>MKRKLFWICAVAMGMSAFPSFMTQATPATQPLINAEPAVAAQTEQNPQVGQVMPGVQGADAPVVAQNGPSRDVKLTFAQIAPPPGSMVLRGINPNGSIEFGMRSDEVVTKAMLNLEYTPSPSLLPVQSQLKVYLNDELMGVLPVTKEQLGKKTLAQMPINPLFITDFNRVRLEFVGHYQDVCENPASTTLWLDVGRSSGLDLTYQTLNVKNDLSHFPVPFFDPRDNRTNTLPMVFAGAPDVGLQQASAIVASWFGSRSGWRGQNFPVLYNQLPDRNAIVFATNDKRPDFLRDHPAVKAPVIEMINHPQNPYVKLLVVFGRDDKDLLQAAKGIAQGNILFRGESVVVNEVKPLLPRKPYDAPNWVRTDRPVTFGELKTYEEQLQSSGLEPAAINVSLNLPPDLYLMRSTGIDMDINYRYTMPPVKDSSRMDISLNNQFLQSFNLSSKQEANRLLLRIPVLQGLLDGKTDVSIPALKLGATNQLRFD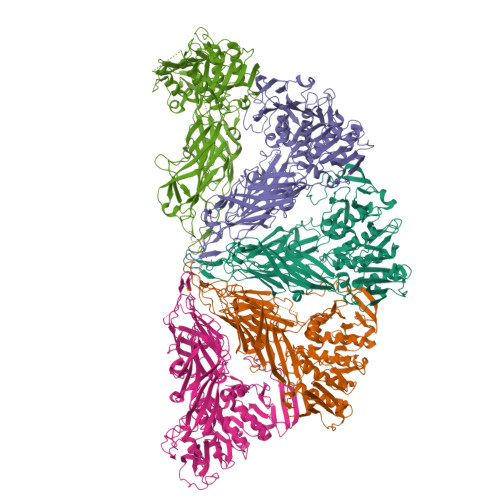FEYMNPMPGGSVDNCITFQPVQNHVVIGDDSTIDFSKYYHFIPMPDLRAFANAGFPFSRMADLSQTITVMPKAPNEAQMETLLNTVGFIGAQTGFPAINLTVTDDGSTIQGKDADIMIIGGIPDKLKDDKQIDLLVQATESWVKTPMRQTPFPGIVPDESDRAAETRSTLTSSGAMAAVIGFQSPYNDQRSVIALLADSPRGYEMLNDAVNDSGKRATMFGSVAVIRESGINSLRVGDVYYVGHLPWFERLWYALANHPILLAVLAAISVILLAWVLWRLLRIISRRRLNPDNE[5x]>GGDRVKKLINSQISLLIGKGLHEFDSLRDPEVNDFRTKMRQFCEEAAAHRQQLGWVEWLQYSFPLQLEPSARGWRAGLLRVSNRALLVNVKFEGSEESFTFQVSTKDMPLALMACALRKKATVFRQPLVEQPEEYALQVNGRHEYLYGNYPLCHFQYICSCLHSGLTPHLTMVHSSSILAMRDEQSNPAPQVQKPRAKPPPIPAKKPSSVSLWSLEQPFSIELIEGRKVNADERMKLVVQAGLFHGNEMLCKTVSSSEVNVCSEPVWKQRLEFDISVCDLPRMARLCFALYAVVEKAKKARSTKKKSKKADCPIAWANLMLFDYKDQLKTGERCLYMWPSVPDEKGELLNPAGTVRGNPNTESAAALVIYLPEVAPHPVYFPALEKILELGRHGERGRITEEEQLQLREILERRGSGELYEHEKDLVWKMRHEVQEHFPEALARLLLVTKWNKHEDVAQMLYLLCSWPELPVLSALELLDFSFPDCYVGSFAIKSLRKLTDDELFQYLLQLVQVLKYESYLDCELTKFLLGRALANRKIGHFLFWHLRSEMHVPSVALRFGLIMEAYCRGSTHHMKVLMKQGEALSKLKALNDFVKVSSQKTTKPQTKEMMHMCMRQETYMEALSHLQSPLDPSTLLEEVCVEQCTFMDSKMKPLWIMYSSEEAGSAGNVGIIFKNGDDLRQDMLTLQMI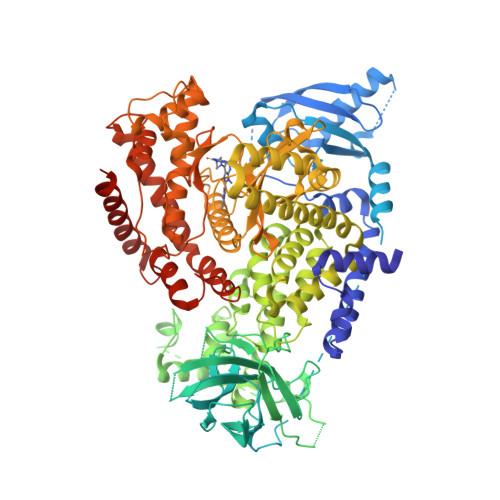QLMDVLWKQEGLDLRMTPYGCLPTGDRTGLIEVVLHSDTIANIQLNKSNMAATAAFNKDALLNWLKSKNPGEALDRAIEEFTLSCAGYCVATYVLGIGDRHSDNIMIRESGQLFHIDFGHFLGNFKTKFGINRERVPFILTYDFVHVIQQGKTNNSEKFERFRGYCERAYTILRRHGLLFLHLFALMRAAGLPELSCSKDIQYLKDSLALGKTEEEALKHFRVKFNEALRESWKTKVNWLAHNVSKDNRQ[2x]> GPDRSFRWKYHQFRFLCHSNALPSHVKISVSRQTLFEDSFQQIMNMKPYDLRRRLYIIMRGEEGLDYGGIAREWFFLLSHEVLNPMYCLFEYAGKNNYCLQINPASSINPDHLTYFRFIGRFIAMALYHGKFIDTGFTLPFYKRMLNKRPTLKDLESIDPEFYNSIVWIKENNLEECGLELYFIQDMEILGKVTTHELKEGGESIRVTEENKEEYIMLLTDWRFTRGVEEQTKAFLDGFNEVAPLEWLRYFDEKELELMLCGMQEIDMSDWQKSTIYRHYTKNSKQIQWFWQVVKEMDNEKRIRLLQFVTGTCRLPVGGFAEL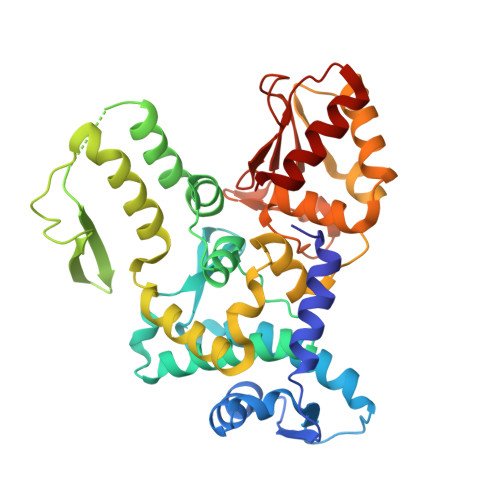IGSNGPQKFCIDKVGKETWLPRSHTCFNRLDLPPYKSYEQLREKLLYAIEETE>[20x]QTDMSRKAFVFPKESDTSYVSLKAPLTKPLKAFTVCLHFYTELSSTRGYSIFSYATKRQDNEILIFWSKDIGYSFTV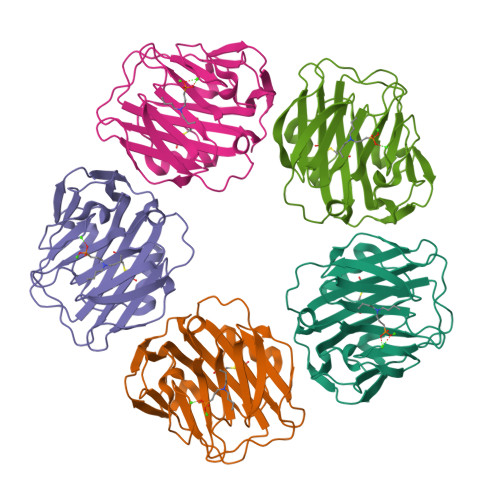GGSEILFEVPEVTVAPVHICTSWESASGIVEFWVDGKPRVRKSLKKGYTVGAEASIILGQEQDSFGGNFEGSQSLVGDIGNVNMWDFVLSPDEINTIYLGGPFSPNVLNWRALKYEVQGEVFTKPQLWP The PBD domain is responsible for the proper cellular localization of Plk1 through an array of phosphorylation-dependent protein–protein interactions mediated by the phosphopeptide-binding groove. Disrupting these interactions has shown potential as a strategy for anticancer therapy. The discovery of an auxiliary flexible pocket on the PBD surface, which is involved in binding a peptide derived from polo-box interacting protein 1 (PBIP1), has been recently reported. Our objective was to prepare more potent ligands of the PBD by improving binding to this auxiliary pocket by optimizing the hydrophobic interactions whilst retaining the key hydrogen bond.

A series of analogues of PBIP1-derived peptide 1 a with phenylalanine replaced by other acetylated hydrophobic and aromatic amino acids (2 a–f) were prepared and tested in the FTS binding mode assay. Interestingly, the pocket turned out to be very specific for hydrophobic aromatic residues. None of tested aliphatic residues (2 a–d) showed ΔΔTm values higher than 1.0 K. To confirm the binding modes, we co-crystallized two representative examples with the PBD, the leucine-based peptide 2 a (ΔΔTm=0.3 K) and the most potent ligand 3 j (ΔΔTm=4.1 K). As predicted, peptide 2 a turned away from the pocket, corroborating the result of the assay.

> GPLGSPEFDCHLSDMLQQLHSVNASKPSERGLVRQEEAEDPACIPIFWVSKWVDYSDKYGLGYQLCDNSVGVLFNDSTRLILYNDGDSLQYIERDGTESYLTVSSHPNSLMKKITLLKYFRNYMSEHLLKAGANITPREGDELARLPYLRTWFRTRSAIILHLSNGSVQINFFQDHTKLILCPLMAAVTYIDEKRDFRTYRLSLLEEYGCCKELASRLRYARTMVDKLLSSR;> XLDPPLHSTAX> ETGMPQYSTFHSENRDWTFNHLTVHRRTGAVYVGAINRVYKLTGNLTI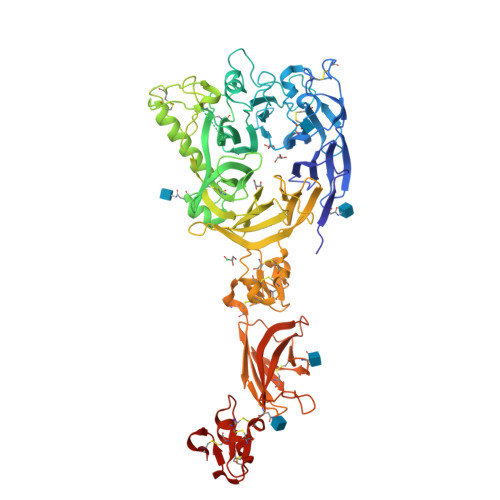QVAHKTGPEEDNKACYPPLIVQPCSEVLTLTNNVNKLLIIDYSENRLLACGSLYQGVCKLLRLDDLFILVEPSHKKEHYLSSVNKTGTMYGVIVRSEGEDGKLFIGTAVDGKQDYFPTLSSRKLPRDPESSAMLDYELHSDFVSSLIKIPSDTLALVSHFDIFYIYGFASGGFVYFLTVQPETPDGMAINSAGDLFYTSRIVRLCKDDPKFHSYVSLPFGCTRAGVEYRLLQAAYLAKPGEALAQAFNISSDEDVLFAIFSKGQKQYHHPPDDSALCAFPIRAINLQIKERLQSCYHGEGNLELNWLLGKDVQCTKAPVPIDDNFCGLDINQPLGGSTPVEGLTLYTTSRDRLTSVASYVYNGYSVVFVGTKSGKLKKIRADGPPHGGVQYEMVSVFKDGSPILRDMAFSINQLYLYVMSERQVTRVPVESCEQYTTCGECLSSGDPHCGWCALHNMCSRRDKCQRAWEANRFAASISQCMSLEVHPNSISVSDHSRLLSLVVNDAPNLSEGIACAFGNLTEVEGQVSGSQVICISPGPKDVPVIPLDQDWFGLELQLRSKETGKIFVSTEFKFYNCSAHQLCLSCVNSAFRCHWCKYRNLCTHDPTTCSFQEGRINVSEDCPQGTKHHHHHH>[2x]GPGSKKFP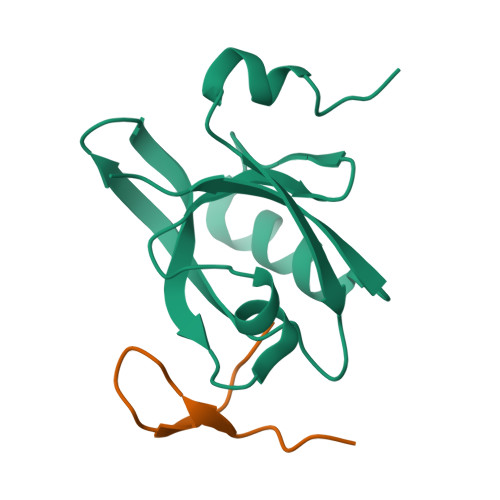TASDETKFIFDQFPKARTVQVRKEGFLGIMVIYGKHAEVGSGIFISDLREGSNAELAGVKVGDMLLAVNQDVTLESNYDDATGLLKRAEGVVTMILLTLK;>GPGSRGKSTVTGRMISGWL[2x]2-cyano-~{N}-(pyridin-4-ylmethyl)ethanamide | C9 H9 N3 O 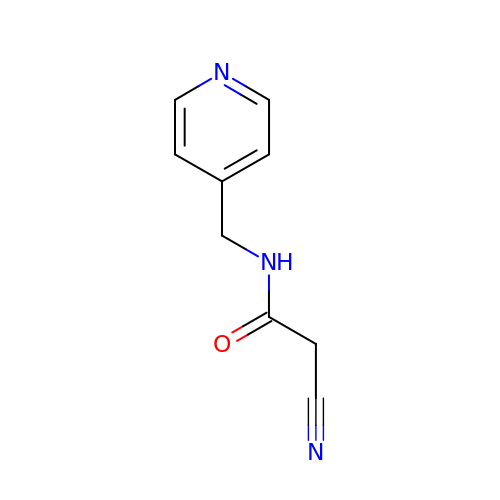| ACPRFCGKSGKRCH-UHFFFAOYSA-N> MAHHGVSGLVGKLVTQLEVNCDADIFYKIVKHHEEVPNVIPHFFTGVQVTKGDGLVSGCIK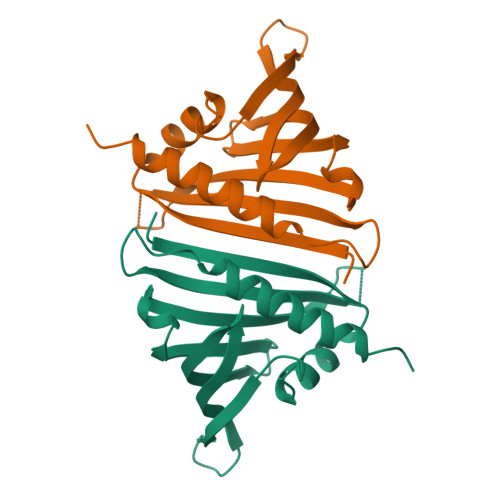EWNYVLEGKAMTAVEETTHADETRTLTHHITEGDAMKDYKKFDVIVETNPKPNGHGSVVTYSIVYEKINEDSPAPFDYLKFFHQNIVDMSAHISSSA>[2x]MVMIESPLLENLTGYIGGRWKDSAGGATFDVYNPATGSVIAKVPSMPEEDVVAAVEAGQSALRLTNPWPIETRRKWLEDIRDGLKENREEIGRILCMEHGKPWK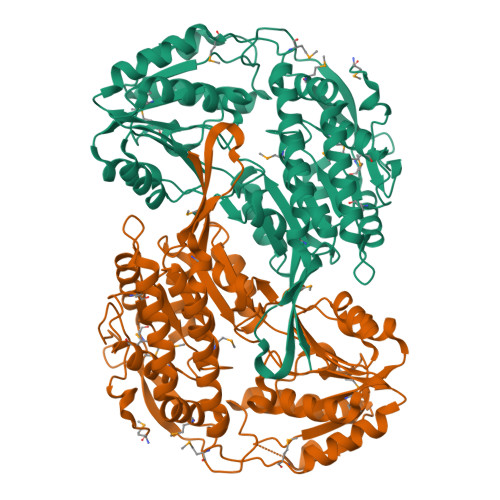EAQGEVDYAAGFFDYCAKHISALDSHTIPEKPKDCTWTVHYRPVGVTGLIVPWNFPIGMIAKKLSAALAAGCPSVIKPASETPLTMIAFFSVMDKLDLPDGMVNLVMGKASVIGKVLCEHKDVPMLSFTGSTEVGRKLIVDTAEQVKKLALELGGNAPFIVFDDADLEAAADNLIANKFRGGGQTCVCANRIFVHEKVADAFGQKLAERVNKMTVGDGMNDGIDIGPLINKQGFDKVKRHLQDALDKGASLVAGKQPAELGDGLFFPPTVVQGVDREMCCYQEETFGPLVPMALFRTEEEVIDAGNDTEFGLASYVFTADAERAQRVAAGLRFGHVGWNTGTGPTPEAPFGGMKASGIGREGGLEGLFEFVEAQTVPRGFAENLYFQSHHHHHHWSHPQFEK> AAMQDRMYQRFLRQHVDPDATGGNDAYCNLMMQRRKMTSHYCKRFNTFIHEDIWNIRSICSTSNIQCKNGQMNCHEGVVKVTDCRETGSSRAPNCRYRAMASTRR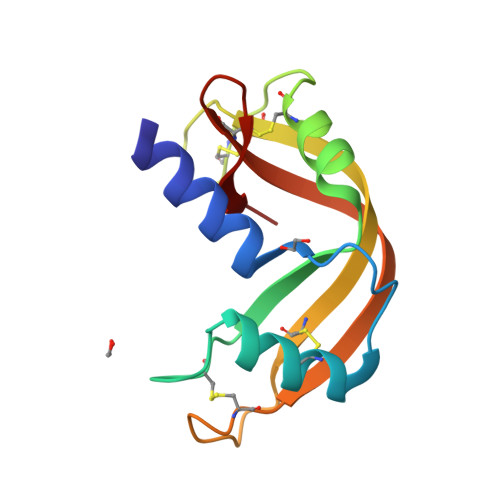VVIACEGNPEVPVHFDK>[2x]GSRRYDVFPSFRGEDVRDSFLSHLLKELRGKAITFIDDEIER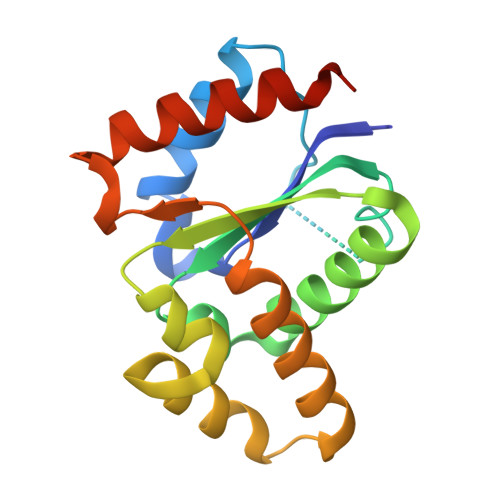SRSIGPELLSAIKESRIAIVIFSKNYASSTWCLNELVEIHKCYTNLNQMVIPIFFHVDASEVKKQTGEFGKVFEETCKAKSEDEKQSWKQALAAVAVMAGYDLRKWPSEAAMIEELAEDVLRKTMTPSDDFG>MGIISYVKKLFKRPAGEIMRMSSGNIGVYKLDDSRVDYELARELYQNKNANYKLGSSFVRPIVNSTTGFMGVPHFQIEDEEAQYILDEFVLDNTSKMLKTHTDSLKQGDCYIWITREERENPLYPDKKVRLIYNFISPEEVKEIILDPTTKEPIAYILESQNEWTDLGENKRKAKVKQIITAESRFVEVEGDKIEGLEEGETPNVWGFIPIIHFKNEADETLKYGQSDIEPIEPLLKAYHDVMLHALKGSKMHSTPKLKLKLTDVASFLAHNFGVEDPVKFAKEGGKINLDGHEILFLNKDEEAEFVEVKSAIGDAKELLKLLFYCIVDVSETPEFIFGVHTPSALASVKEQMPIMVNKIRRKREQFTNSWQLLARMVLIMSSNSSGMKYSSYDVTIGWDEVNPRDDKELAETLEKVCCALDKALEGGFISEESTVNFLAQYIDTMSN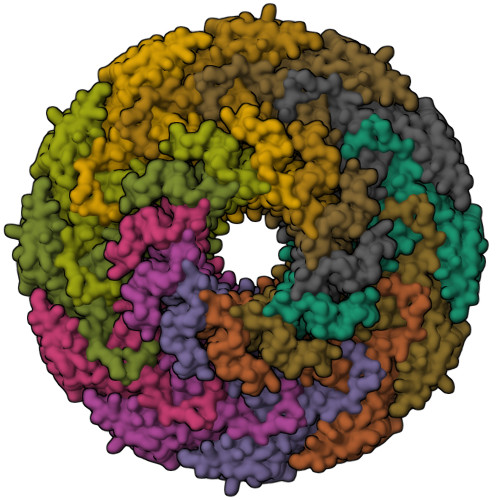YISDDPEREGEREKIIKTKMLKYRLDDSQGLNDESNEIEKEINKIKDNNGNG[12x]>SNAMTGLFVTLEGPEGAGKSTNRDYLAERLRERGIEVQLTREPGGTPLAERIRELLLAPSDEPMAADTELLLMFAARAQHLAGVIRPALARGAVVLCDRFTDATYAYQGGGRGLPEARIAALESFVQGDLRPDLTLVFDLPVEIGLARAAARGRLDRFEQEDRRFFEAVRQTYLQRAAQAPERYQVLDAGLPLAEVQAGLDRLLPNLLERLNG[4x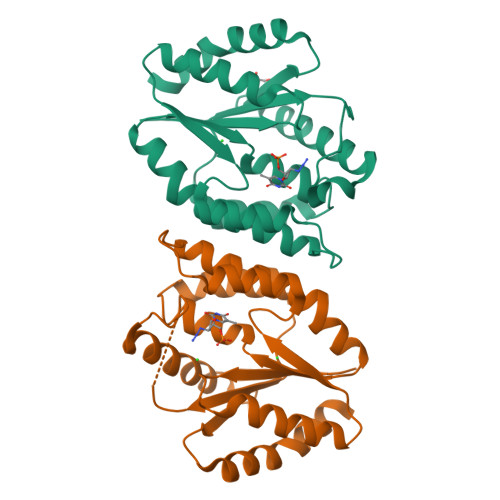]>MVHHHHHHNEDICFIAGIGDTNGYGWGIAKELSKRNVKIIFGIWPPVYNIFMKNYKNGKFDNDMIIDKDKKMNILDMLPFDASFDTANDIDEETKNNKRYNMLQNYTIEDVANLIHQKYGKINMLVHSLANAKEVQKDLLNTSRKGYLDALSKSSYSLISLCKYFVNIMKPQSSIISLTYHASQKVVPGYGGGMSSAKAALESDTRVLAYHLGRNYNIRINTISAGPLKSRAATAINKLNNTYENNTNQNKNRNSHDVHNI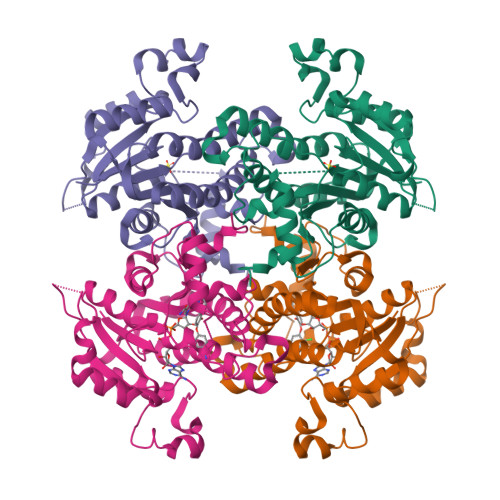MNNSGEKEEKKNSASQNYTFIDYAIEYSEKYAPLRQKLLSTDIGSVASFLLSRESRAITGQTIYVDNGLNIMFLPDD[2x]> XGGCUUGCA;> GGUCCGCA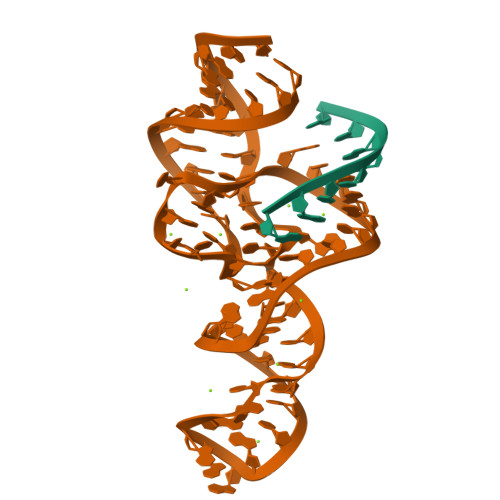GCCUCCUCGCGGCGCAAGCUGGGCAACAUUCCGAAAGGUAAUGGCGAAUGCGGACC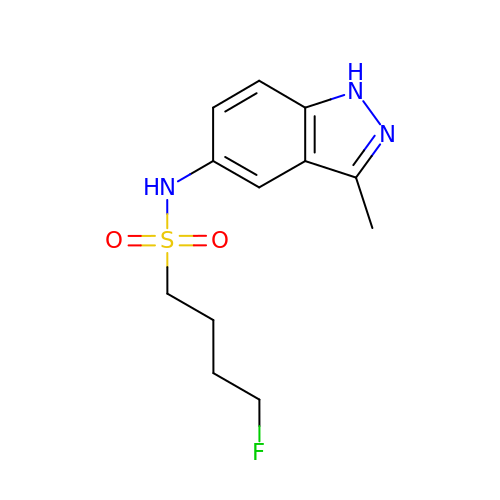4-fluoro-N-(3-methyl-1H-indazol-5-yl)butane-1-sulfonamide | C12 H16 F N3 O2 S | AHVAAGWAEHSRBU-UHFFFAOYSA-N>[16x]MHHHHHHSLTDLVEQPAKVMRIGTMIKQLLEEVRAAPLDEASRNRLRDIHATSIRELEDGLAPELREELDRLTLPFNED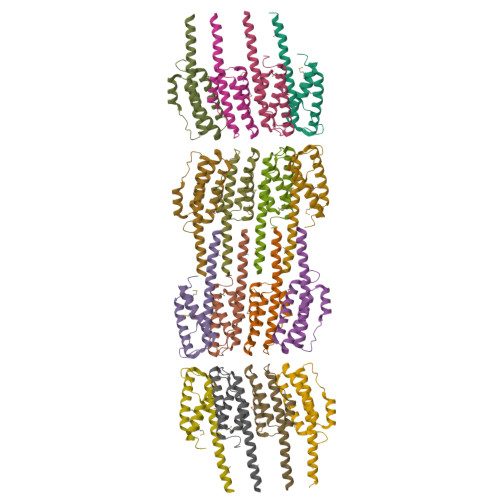AVPSDAELRIAQAQLVGWLEGLFHGIQTALFAQQMAARAQLQQMRQGALPPG{(2R,4E)-2-(hydroxymethyl)-4-[5-methyl-3-(2-methylpropyl)hexylidene]-5-oxooxolan-2-yl}methyl 2,2-dimethylpropanoate | C22 H38 O5 | 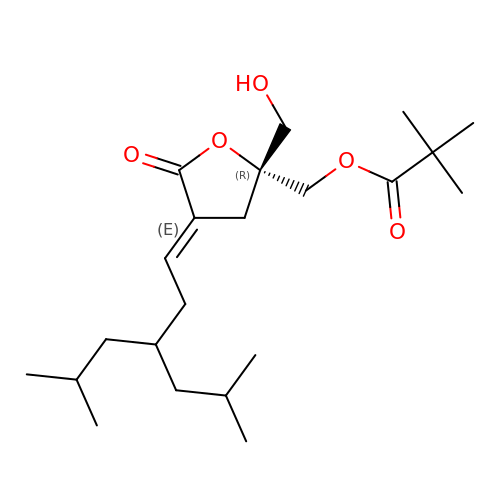XKEOGEXDEKIDNA-XROMRFNBSA-N>[3x]MGDSEEPVVTPHAPEFAFDPTDPWTETFQRGLEIAGLGGKRVYEVGIGTGINVAFMLQICEAALVSGSDLDPRLAGLAERNVRDLAPRRADRFHPVEGAVSLIDTPEARAQVGRSDVIVGCLPQVGEPDDVRLRAFRTAQAAALAAGADTRDEDHIAHYYPWAEFDSYPFNSVGLGLNEALLRRTRATAPAADVVLN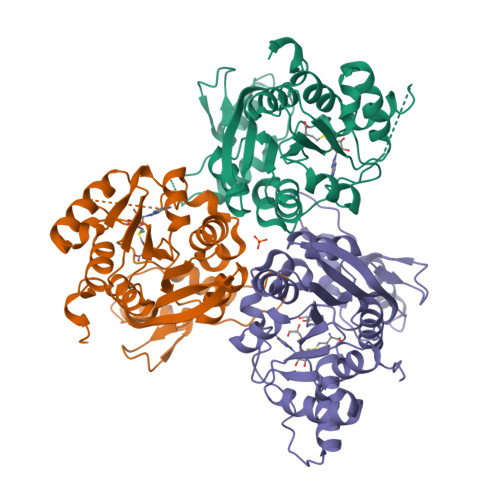FGARVGSAVLFELFEANGYVPEKLHSQIVLQHAGTDISFFVALENALAQTGLEREFTCEFYGDPEGATRLSATEAQALVDTDSAAEIYHEVCVIRGRPALSENDPSDS MtbTOP1 and topoisomerase I present in all bacterial pathogens are type IA topoisomerases that are needed for resolving topological barriers that require the passage of DNA through the break created on single-stranded DNA (ssDNA). M. tuberculosis topoisomerase I (MtbTOP1) is a validated target for much needed new antibiotics that can be used against the MDR-TB (multidrug-resistant tuberculosis) cases that are difficult to treat (1–3). The MtbTOP1-704t construct includes four N-terminal domains (D1–D4) and one C-terminal domain (D5). D1–D4 form a toroidal assembly found in all topoisomerase IA while D5 represents the Topo_C_Rpt subgroup of bacterial topoisomerase C-terminal repeats.

No significant conformational change has been observed among these structures even though they have different crystal symmetries. This indicates that the N-terminal toroidal assembly of the enzyme is quite stable by itself.

>SNAADPKTKGRGSGGNGSGRRLVIVESPTKARKLASYLGSGYIVESSRGHIRDLPRAASDVPAKYKSQPWARLGVNVDADFEPLYIISPEKRSTVSELRGLLKDVDELYLATDGDREGEAIAWHLLETLKPRIPVKRMVFHEITEPAIRAAAEHPRDLDIDLVDAQETRRILDRLYGYEVSPVLWKKVAPKLSAGRVQSVATRIIVARERDRMAFRSAAYWDILAKLDASVSDPDAAPPTFSARLTAVAGRRVATGRDFDSLGTLRKGDEVIVLDEGSATALAAGLDGTQLTVASAEEKPYARRPYPPFMTSTLQQEASRKLRFSAERTMSIAQRLYENGYITYMRTDSTTLSESAINAARTQARQLYGDEYVAPAPRQYTRKVKNAQEAHEAIRPAGETFATPDAVRRELDGPNIDDFRLYELIWQRTVASQMADARGMTLSLRITGMSGHQEVVFSATGRTLTFPGFLKAYVETVDELVGGEADDAERRLPHLTPGQRLDIVELTPDGHATNPPARYTEASLVKALEELGIGRPSTYSSIIKTIQDRGYVHKKGSALVPSWVAFAVTGLLEQHFGRLVDYDFTAAMEDELDEIAAGNERRTNWLNNFYFGGDHGVPDSVARSGGLKKLVGINLEGIDAREVNSIKLFDDTHGRPIYVRVGKNGPYLERLVAGDTGEPTPQRANLSDSITPDELTLQVAEELFAT[2x]> ESDTGLWLHNKLGATDELWAPPSIASLLTAAVIDNIRLCFHGLSSAVKLKLLLGTLHLPRRTVDEMKGALMEIIQLASLDSDP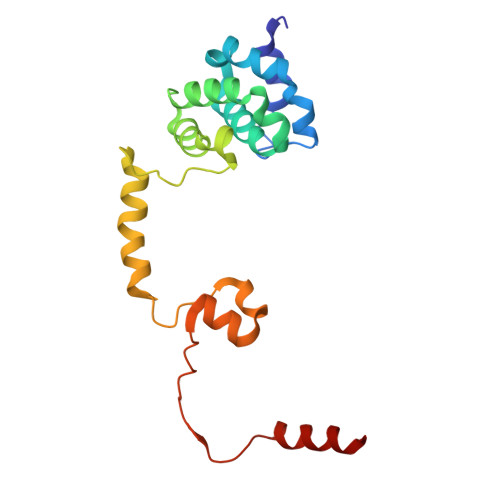WVLMVADILKSFPDTGSLNLELEEQNPNVQDILGELREKVGECEASAMLPLECQYLNKNALTTLAGPLTPPVKHFQLKRKPKSATLRAELLQKS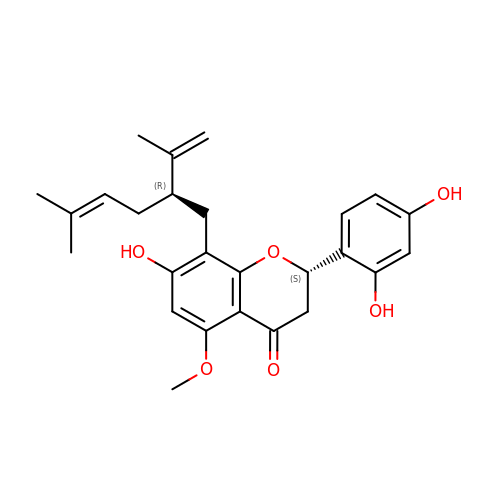(2S)-2-[2,4-bis(oxidanyl)phenyl]-5-methoxy-8-[(2R)-5-methyl-2-prop-1-en-2-yl-hex-4-enyl]-7-oxidanyl-2,3-dihydrochromen-4-one | C26 H30 O6 | LTTQKYMNTNISSZ-MWTRTKDXSA-N>MAFKVISQENLLEQKRKETLQEDIPFIVNGEMEYVTKKISNGEMETLELNKPLGEMMTFSSTSNLKELLRKVVLDVELGREQVQLLYKPIYDSIADSNLPQVMDAKWALQGNCVFLEHIEGEEIKFGTINAENGPVARIQTYATGFEYTKEMKDFNQTFSVEILNKSIGESYNALLNHIHLSPIINFNYKASNKTAFKGETNDPIWLGIWRTLTQAQKDTVIAKRQGNILMASSADQIEIEMALNGGHLLNGSMYPSIKNISTVIYYDGWEVTVGKKTYSYKGVTPGKGYLIRPKRGFKELIKRDLTTEVGNADLSKLVENQIVGHCYRGAFAAVEENVQEISFR[7x];>MAFKGQPTPSTITQITRAKISDGKSVRVILSEGESTKTQQFYLINGFFGVAMQDGEKGDEVTLQIEQAEYETDNIVTSEAFEAGKLIYWDNTAKKFTTTSASNRLVGRVTDGKDSNNVIWFILLPQQ[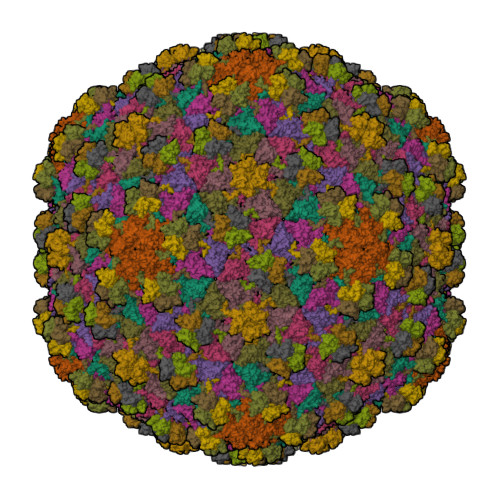7x]>[2x]PRGSHMIILAFDIFGTVLDTSTVIQEFRNKQLEYTWLLT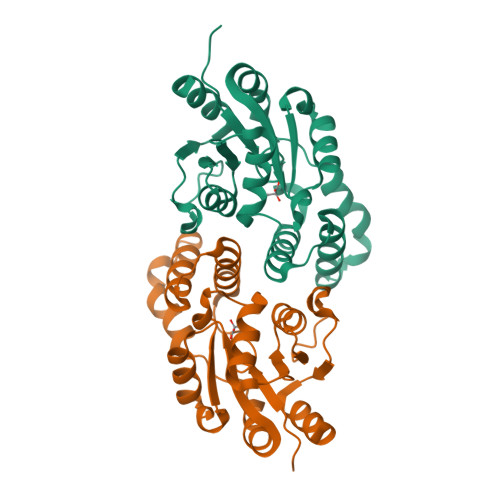IMGKYVEFEEITKITLRYILKVRGEESKFDEELNKWKNLKAYEDTKYLKEISEIAEVYALSNGSINEVKQHLERNGLLRYFKGIFSAESVKEYKPSPKVYKYFLDSIGAKEAFLVSSNAFDVIGAKNAGMRSIFVNRKNTIVDPIGGKPDVIVNDFKELYEWILRYK>TNSAGIAQQWIQSKREDIVNQMTEACLNQSLDALLSRDLIMKEDYELVSTKPTRTSKVRQLLDTTDIQGEEFAKVIVQKLKDNKQMGLQPYPEILVVSRSPSLNLLQNKSM[12x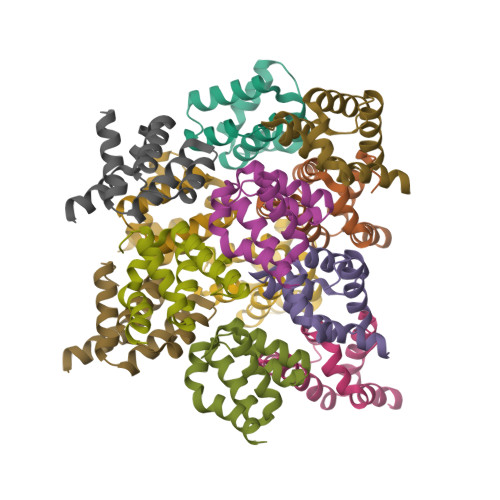]> ADPKKVLDKAKDQAENRVRELKQKLEELYKEARKLDLTQEMRRKLELRYIAAMLMAIGDIYNAIRQAKQEADKLKKAGLVNSQQLDELK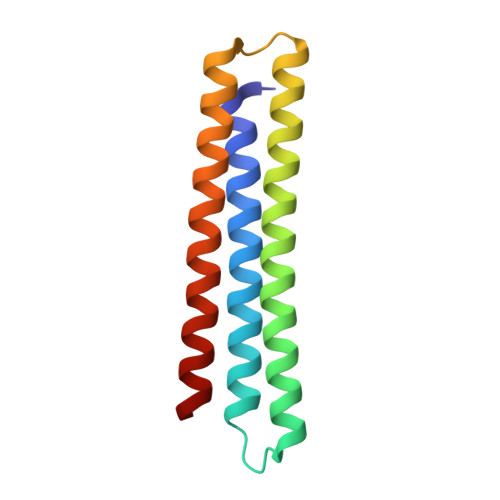RRLEELKEEASRKARDYGREFQLKLEYG>MKFRRSGRLVDLTNYLLTHPHELIPLTFFSERYESAKSSISEDLTIIKQTFEQQGIGTLLTVPGAAGGVKYIPKMKQAEAEEFVQTLGQSLANPERILPGGYVYLTDILGKPSVLSKVGKLFASVFAEREIDVVMTVATKGIPLAYAAASYLNVPVVIVRKDNKVTEGSTVSINYVSGSSNRIQT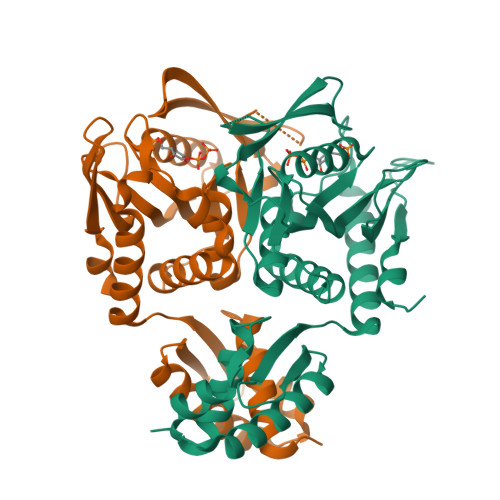MSLAKRSMKTGSNVLIIDDFMKAGGTINGMINLLDEFNANVAGIGVLVEAEGVDERLVDEYMSLLTLSTINMKEKSIEIQNGNFLRFFKDNLLKNGETES[4x]>MKNVGFIGWRGMVGSVLMQRMVEERDFDAIRPVFFSTSQLGQAAPSFGGTTGTLQDAFDLEALKALDIIVTCQGGDYTNEIYPKLRESGWQGYWIDAASSLRMKDDAIIILDPVNQDVITDGLNNGIRTFVGGNCTVSLMLMSLGGLFANDLVDWVSVATYQAASGGGARHMRELLTQMGHLYGHVADELATPSSAILDIERKVTTLTRSGELPVDNFGVPLAGSLIPWIDKQLDNGQSREEWKGQAETNKILNTSSVIPVDGLCVRVGA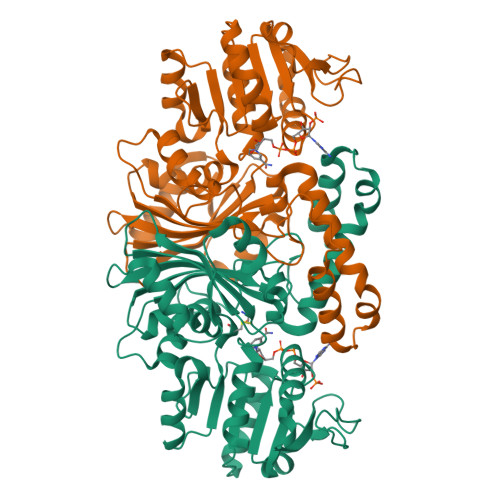LRCHSQAFTIKLKKDVSIPTVEELLAAHNPWAKVVPNDREITMRELTPAAVTGTLTTPVGRLRKLNMGPEFLSAFTVGDQLLWGAAEPLRRMLRQLA[2x]>[2x]MSISTSAEVYYEEAEEFLSKGDLVQACEKYYKAAEEAIKLLVIENNLKEITNNVKNKGRWKSENLFKASKLLRSNNTEIPILWKSAWTLHVEGFHELSLNEKEVKKLKEDVRKLVIFA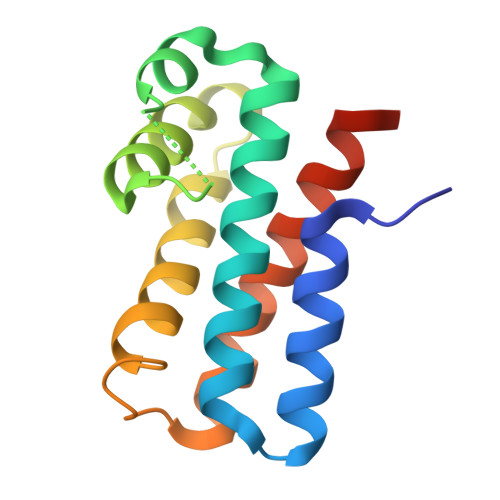VNSLEHHHHHH> AVPCVSGGLPKPANI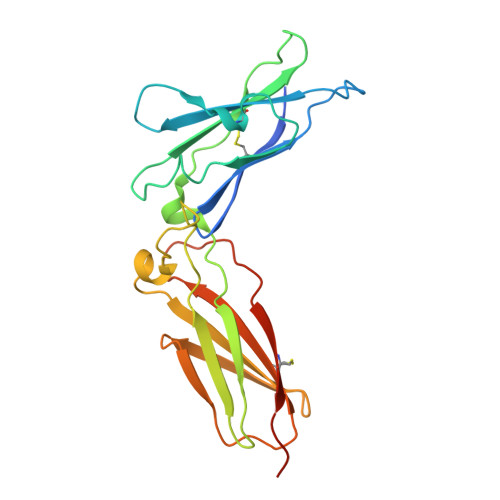TFLSINMKNVLQWTPPEGLQGVKVTYTVQYFIYGQKKWLNKSECRNINRTYCDLSAETSDYEHQYYARVRAIWGTKCSKWAESGRFYPFLETQIGPPEVALTTDEKSISVVLTAPEKWKRNPEDLPVSMQQIYSNLKYNVSVLNTKSNRTWSQCVTNHTLVLTWLEPNTLYCVHVESFVPGPPRRAQPSEKQCARTLKDQSSIEGR> NSSTASKTYNYVYSSDPSSLNYLAENRAATSDIVANLVDGLLENDQYGNIIPSLAEDWTVSQDGLTYTYKLRKDAKWFTSEGEEYAPVTAQDFVTGLQYAADKKSEALYLVQDSVAGLDDYITGKTSDFSTVGVKALDDQTVQYTLVKPELYWNSKTLATILFPVNADFLKSKGDDFGKADPSSILYNGPFLMKALVSKSAIEYKKNPNYWDAKNVFVDDVKLTYYDGSDQESLERNFTAGAYTTARLFPNSSSYEGIKEKYKNNIIYSMQNSTSYFFNFNLDRKSYNYTSKTSDIEKKSTQEAVLNKNFRQAINFAFDRTSYGAQSEGKEGATKILRNLVVPPNFVSIKGKDFGEVVASKMVNYGKEWQGINFADGQDPYYNPEKAKAKFAEAKKELEAKGVQFPIHLDKTVEVTDKVGIQGVSSIKQSIESVLGSDNVVIDIQQLTSDEFDSSGYFAQTAAQKDYDLYHGGWGP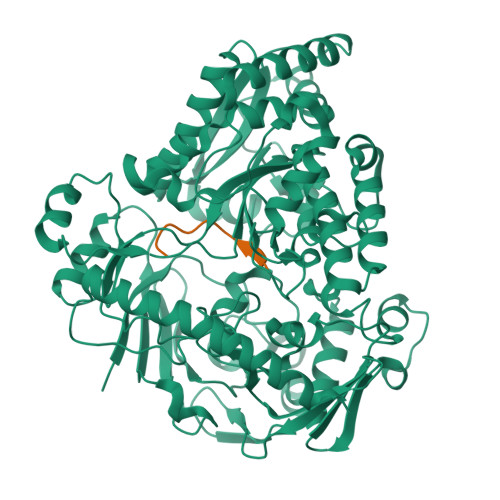DYQDPSTYLDIFNTNSGGFLQNLGLEPGEANDKAKAVGLDVYTQMLEEANKEQDPAKRYEKYADIQAWLIDSSLVLPSVSRGGTPSLRRTVPFAAAYGLTGTKGVESYKYLKVQDKIVTTDEYAKAREKWLKEKEESNKKAQEELAKHVK> GHMAVIKVIGVGGGGGNAVEHMVRERIEGVEFFAVNTDAQALRKTAVGQTIQIGSGITKGLGAGANPEVGRNAADEDREALRAALDGADMVFIAAGMGGGTGTGAAPVVAEVAKDLGILTVAVVTKPFNFEGKKRMAFAEQGITELSKHVDSLITIPNDKLLKVLG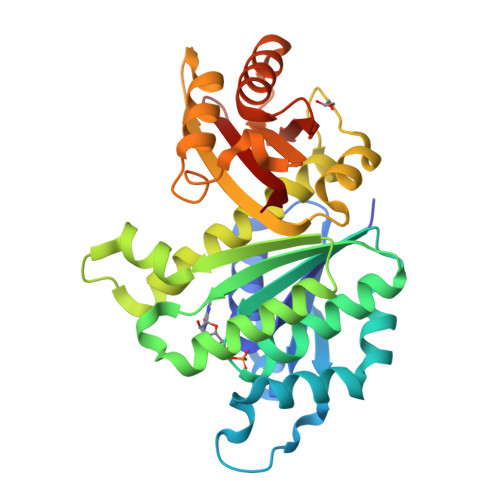RGISLLDAFGAANDVLKGAVQGIAELITRPGLMNVDFADVRTVMSEMGYAMMGSGVASGEDRAEEAAEMAISSPLLEDIDLSGARGVLVNITAGFDLRLDEFETVGNTIRAFASDNATVVIGTSLDPDMNDELRVTVVATGIG> MG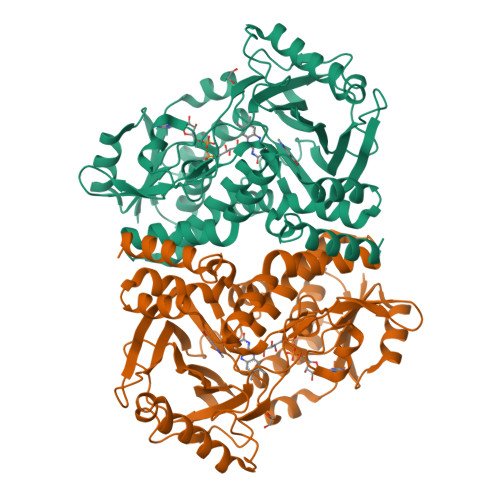HHHHHHHHHHSSGHIEGRHMKRIAIVGAGQSGLQLGLGLLAAGYEVTMFSNRTGEDIRRGKVMSSQCMFDTSLQIERDLGLDHWASDCPTVDGIGLAVPHPEQKGAKVIDWAARLNASAQSVDQRLKIPAWMDEFQKKGGELVFKDAGIDELEACTQSHDLTLVASGKGEISKLFERDAHKSPYDKPQRALALTYVKGMAPREPFSAVCMNLIPGVGEYFVFPALTTTGPCEIMVFEGVPGGPMDCWADVKTPEEHLARSKWILDTFTPWEAERCKDIELTDDNGILAGRFAPTVRKPVATLPSGRKVLGLADVVVLNDPITGQGSNNAAKCADTYLKSILARGDGAADAAWMQQTFDRYWFGYAQWVTQWTNMLLAPPPPHVLNLLGSAGAVPPLASAFANGFDDPRTFFPWFADAAESERYIATCAAVA>MVRPSFSSIVEVKIGGAKLPDTIAPMLTDGWVDQGVNVPAAFRLTFRDPYHRLLGDLNVQFGTKVVITPIADGQGKNNPLLTGEVTGLETDYDGTGSFTVIRGYDYGHRLMRQRRVAAYRNQKASDIARKLVQMDGVSVGRIQPTKGTYAFIAQPNVTDWDFLARLADENKMIMYLDSKGKFRFVTPKPSAGAPSPNTDGDQSAFVLQAGHDILRLRAAVTAADQIGKVESRGWNVTTKKKITEIAPATTDPGISIKWTPGTAAGKFKPGKLVETANPYDKQDEVQNAAKALASDVTASFSELEVAANGHPDLRPGVPVALSDVGTPFEGKYTVTSVRHHFGDGVAYESWITVSGRQWRSLYGLASGGGGSDPASATRLPSVANAIVTDVQDPLKQGRVKLQFPWLDDTYVSDWARSVQMGGVAGGGIFPMDVGDEVLVAFDRGALDHPFVIGGLYNGRDVPTKSDVPLHDGLKKKAVRHTLSDRQGNRVDLLSQRTGGRKQGVRIASGNDKLTINLDRTKTEITVDSKGSVSITGSRSVSVDAGTDLSLSARRSLTIKSGGPLSIQGGSTINMRSGGLVGVNAGGALNLGAGGAATLSAGAATTISGTVNVQINSVMTRVIGATFEVKTPIFKVATIPVPGL[3x]

Bacterial contractile injection systems (CIS) are phage tail-like macromolecular complexes that mediate cell-cell interactions by injecting effector proteins into target cells. Using Streptomyces coelicolor as a model organism, we and others previously demonstrated that S. coelicolor CIS (CISSc) mediate a form of regulated cell death, which influences the onset of sporulation and secondary metabolite production in response to exogenous stress and unknown cellular signals (Casu et al., 2023; Vladimirov et al., 2023). The purified assemblies were subjected to single-particle cryo-electron microscopy (cryoEM) for structure determination, yielding the first high-resolution model of the CISSc in its extended conformation, which also presents the first example of a CIS IId subtype. Our model shows that extended CISSc particles share the conserved eCIS architecture, including the three core modules: cap, sheath tube, and baseplate.

The baseplate module comprises a heteromeric assembly of the proteins Cis1b/7/8/9/11/12. The symmetry transition from the inner tube (Cis1a, C6) to the VgrG-like spike (Cis8, C3) is adapted by two layers of the tube initiators Cis1b and Cis7. (a–f) Local resolution maps of the CISSc baseplate with C6 symmetry (a), CISSc baseplate with C3 symmetry (c), and the CISSc cap with C6 symmetry (e).Sacubitrilat | C22 H25 N O5 | 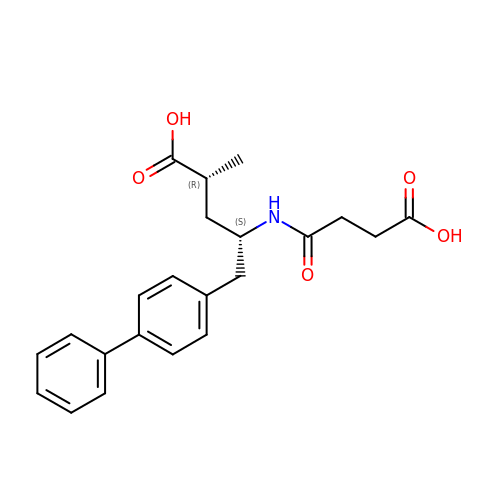DOBNVUFHFMVMDB-BEFAXECRSA-N>GGGGGGMKLFKELEETKEQVIKMAKLVQEAIDKATEALNKQNVELAEEVIKGDDTIDLLEVDIERRCIRMIALYQPEAGDLRMIMGIYKIVSDLERMGDEAENIAERAILLAEEPPLKPYVNINFMSEIVKEMVNDSVISFIQQDTLLAKKVIEKDDTVDELYHQLERELMTYVLEDPRNIKRAMHLS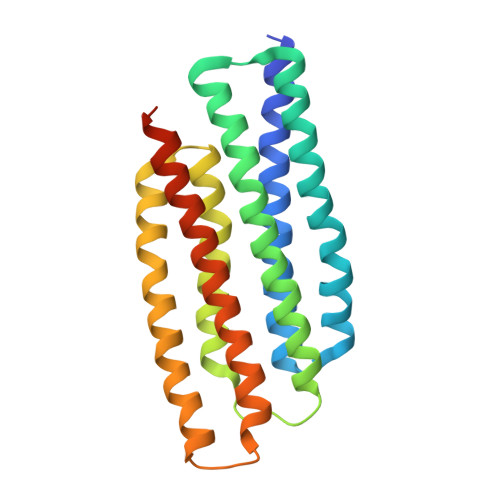FVARHYERIADHAENVAEAAIYLSEGEIVKHQHIKEKGE[2x]> GPVCAEASDVYSPCMIASTPPAPFSDVTAVTFDLINGKITPVGDDNWNTHIYNPPIMNVLRTAAWKSGTIHVQLNVRGAGVKRADWDGQVFVYLRQSMNPESYDARTFVISQPGSAMLNFSFDIIGPNSGFEFAESPWANQTTWYLECVATNPRQIQQFEVNMRFDPNFRVAGNILMPPFPLSTETPPL;> MEQNLFALSLDDTSSVRGSLLDTKFAQTRVLLSKAMAGGDVLLDEYLYDVVNGQDFRATVAFLRTHV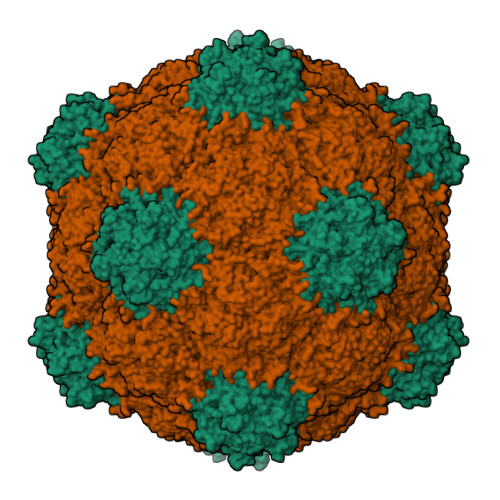ITGKIKVTATTNISDNSGCCLMLAINSGVRGKYSTDVYTICSQDSMTWNPGCKKNFSFTFNPNPCGDSWSAEMISRSRVRMTVICVSGWTLSPTTDVIAKLDWSIVNEKCEPTIYHLADCQNWLPLNRWMGKLTFPQGVTSEVRRMPLSIGGGAGATQAFLANMPNSWISMWRYFRGELHFEVTKMSSPYIKATVTFLIAFGNLSDAFGFYESFPHRIVQFAEVEEKCTLVFSQQEFVTAWSTQVNPRTTLEADGCPYLYAIIHDSTTGTISGDFNLGVKLVGIKDFCGIGSNPGIDGSRLL>[2x]TGEEVLWHTSVPFAENMSLECVYPSMGI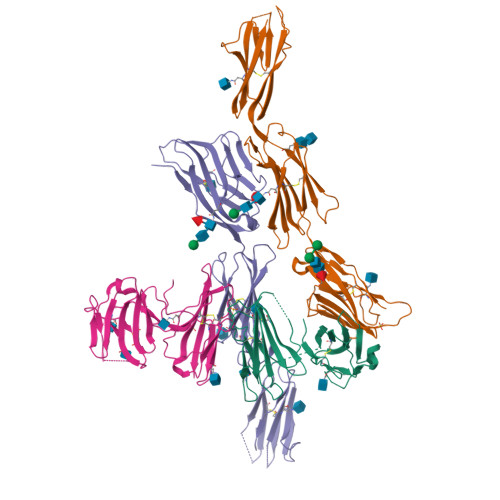LTQVEWFKIGTQQDSIAIFSPTHGMVIRKPYAERVYFLNSTMASNNMTLFFRNASEDDVGYYSCSLYTYPQGTWQKVIQVVQSDSFEAAVPSNSHIVSEPGKNVTLTCQPQMTWPVQAVRWEKIQPRQIDLLTYCNLVHGRNFTSKFPRQIVSNCSHGRWSVIVIPDVTVSDSGLYRCYLQASAGENETFVMRLTVAEGKTDNQYTGTKHHHHHH;>LEDVVVQAPTQVPGFLGDSVTLPCYLQVPNMEVTHVSQLTWARHGESGSMAVFHQTQGPSYSESKRLEFVAARLGAELRNASLRMFGLRVEDEGNYTCLFVTFPQGSRSVDIWLRVLAKPQNTAEVQKVQLTGEPVPMARCVSTGGRPPAQITWHSDLGGMPNTSQVPGFLSGTVTVTSLWILVPSSQVDGKNVTCKVEHESFEKPQLLTVNLTVYYPPEVSISGYDNNWYLGQNEATLTCDARSNPEPTGYNWSTTMGPLPPFAVAQGAQLLIRPVDKPINTTLICNVTNALGARQAELTVQVKEGPPTSHHHHHH[2x]> MSSEANPPVLEPFTVTVVDRNVKHQVEGEPEEEGHPDHEVQGVMFATNVKYIFEDDQELLPEQEDPAIENVVIIEADESLRVT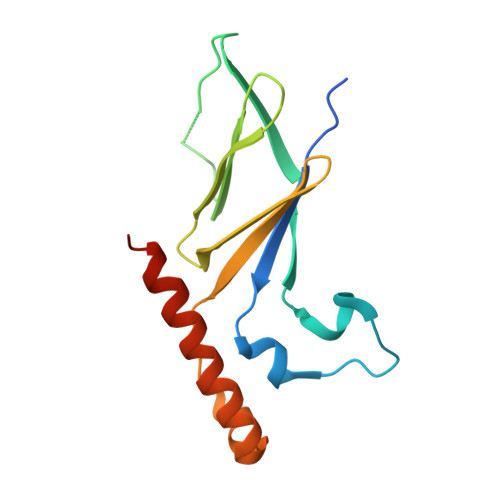QVELISDQFKQVGYEVRDGNEVCIDALSRFETPRQLGNLPLEKLVQLYKLQNDQLHSLFNTLHHHHHH>[4x]MSSLSRELVFLILQFL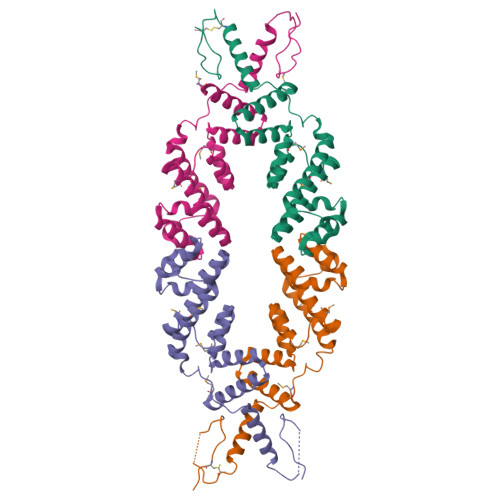DEEKFKETVHKLEQESGFFFNMKYFEEKVHAGEWDEVEKYLSGFTKVDDNRYSMKIFFEIRKQKYLEALDRHDRAKAVDILVKDLKVFSTFNEELYKEITQLLTLENFRENEQLSKYGDTKSARSIMLIELKKLIEANPLFREKLVFPTLKASRLRTLINQSLNWQHQLCKNPRPNPDIKTLFTDHTCTPPNG>SLRSDLINALYDENQKYDVCGIISAEGKIYPLGSDTKVLSTIFELFSRPIINKIAEKHGYIVEEPKQQNHYPDFTLYKPSEPNKKIAIDIKATYTNKENEKIKFTLGGYTSFIRNNTKNIVYPFDQYIAHWIIGYVYTRVATRKSSLKTYNINELNEIPKPYKGVKVFLQDKWVIAGDLAGSGNTTNIGSIHAHYKDFVEGKGIFDSEDE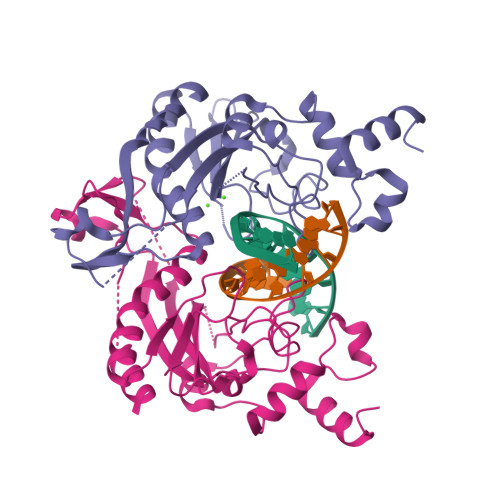FLDYWRNYERTSQLRNDKYNNISEYRNWIYRGRK[2x]> KYNLKMGM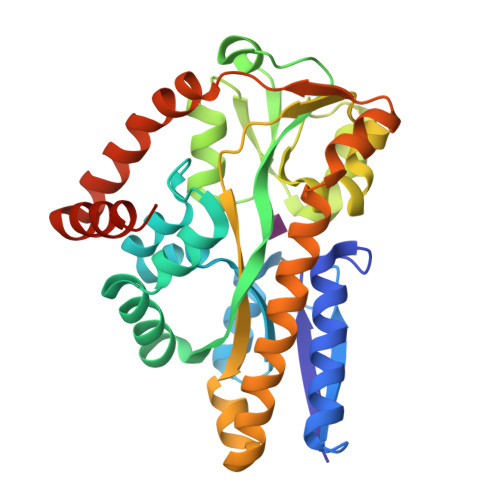TAGTSQNEYKAAEVFAKELKKRSNGEIELKLYPNAQLGKDDLAMMQQLEGGALDFTFAETGRFSTFFPEAEVFTLPYMIKDFNHMKKAVNTKFGKDLFKKVHDKKGMTVLAQAYNGTRQTTSNKAIKSLADMKGMKLRVPGAAANLAYAKYTEAAPTPMAFSEVYLALQTNAVDGQENPLSTIKAQKFYEVQKYLAMTNHILNDQLYLVSNITMEELPENLQKVVKESAEVAAEYHTKLFMDEEKSLKDFFKSKGVTITEPNLVDFKKAMKPFYDEYIKKNGKVGENAIKAIEAVRLEHHHHHH5-[(3aS,4S,6aR)-1-acetyl-2-oxohexahydro-1H-thieno[3,4-d]imidazol-4-yl]pentanoic acid 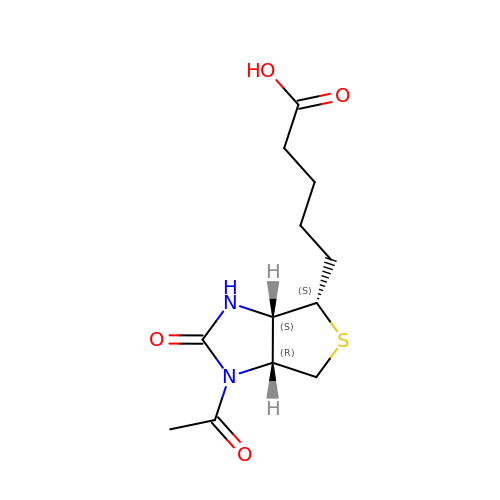| C12 H18 N2 O4 S | LXKFOEIWWHPOIN-QXEWZRGKSA-N>ADRADILY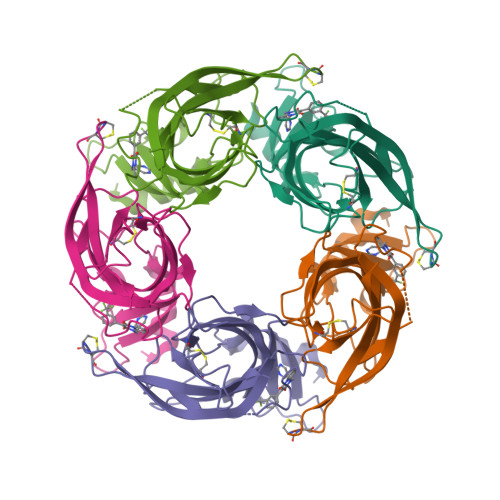NIRQTSRPDVIPTQRDRPVAVSVSLKFINILEVNEITNEVDVVFWQRTTWSDRTLAWDSSHSPDQVSVPISSLWVPDLAAYNAISKPEVLTPQLARVVSDGEVLYVPSIRQRFSCDVSGVDTESGATCRIKIGSWTHHSREISVDPTTENSDDSEYFSQYSRFEILDVTQKKNSVTYSCCPEAYEDVEVSLNFRKKGRSEIL[5x]> MELL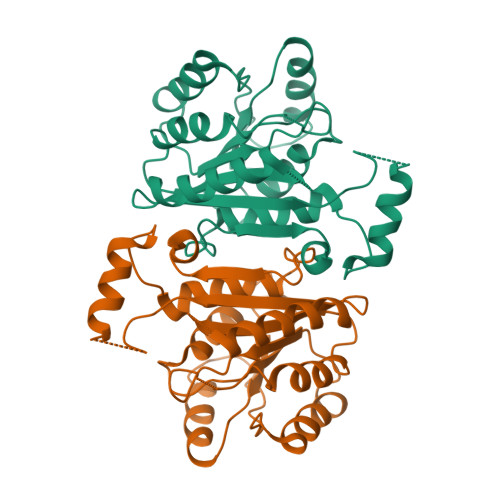QGKTFVVMGVANQRSIAWGIARSLHNAGAKLIFTYAGERLERNVRELADTLEGQESLVLPCDVTNDEELTACFETIKQEVGTIHGVAHCIAFANRDDLKGEFVDTSRDGFLLAQNISAFSLTAVAREAKKVMTEGGNILTLTYLGGERVVKNYNVMGVAKASLEASVKYLANDLGQHGIRVNAISAGPIRTLSAKGVGDFNSILREIEERAPLRRTTTQEEVGDTAVFLFSDLARGVTGENIHVDSGYHILG> MKSIAALLALASAAAAFTPQSQSTSSTALKERISPLDPSIGVTEPLGLYDPLGWLDPEKDPASKFATFHANFERRRAVERKHGRIAMVAVVGMLFHNADIEFPGYLSKELGIRFSDVPNGMNGLFSIPLAGLTQIVFAIGVM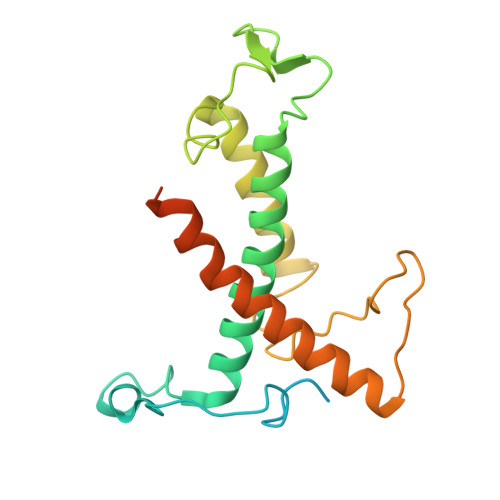ELAIWPASNYSGDYGTGYGRPFVPNVLEGDELKYKLDMEINQGRAAMMGIMGALVGEAVTGQTLAEQIASNNLGLFSALFE> EDGGSWKYPDAF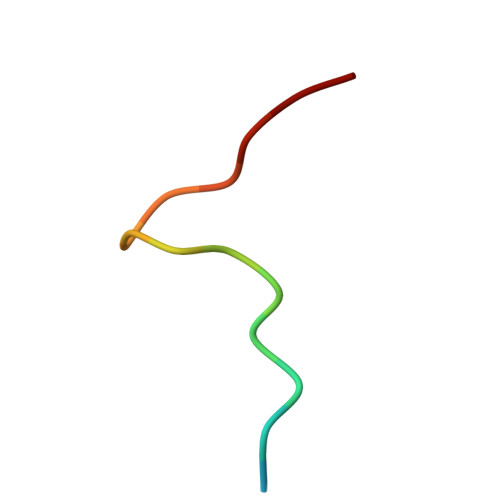ELSG> SH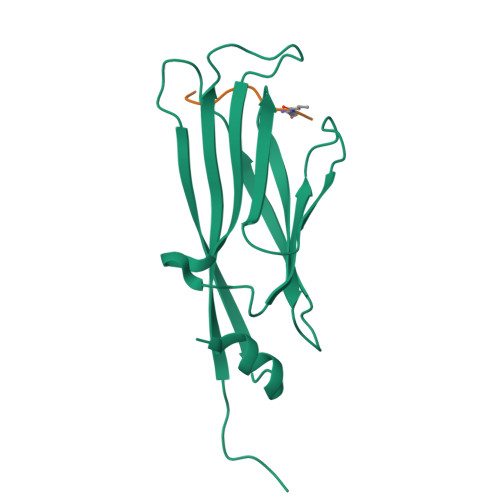MASSCAVQVKLELGHRAQVRKKPTVEGFTHDWMVFVRGPEHSNIQHFVEKVVFHLHESFPRPKRVCKDPPYKVEESGYAGFILPIEVYFKNKEEPRKVRFDYDLFLHLEGHPPVNHLRCEKLTFNNPTEDFRRKLLKA;> TKQTARXS> GPGYNEPMAASDEVNLIESRTVVPLNTWVLISNFKVAYNILRRPDGTFNRHLAEYLDRKVTANANPVDGVFSFDVLIDRRINLLSRVYRPAYADQEQPPSILDLEKPVDGDIVPVILFFHGGSFAHSSANSAIYDTLCRRLVGLCKCVVVSVNYRRAPENPYPCAYDDGWIALNWVNSRSWLKSKKDSKVHIFLAGDSSGGNIAHNVALRAGESGIDVLGNILLNPMFGGNERTESEKSLDGKYFVTVRDRDWYWKAFLPE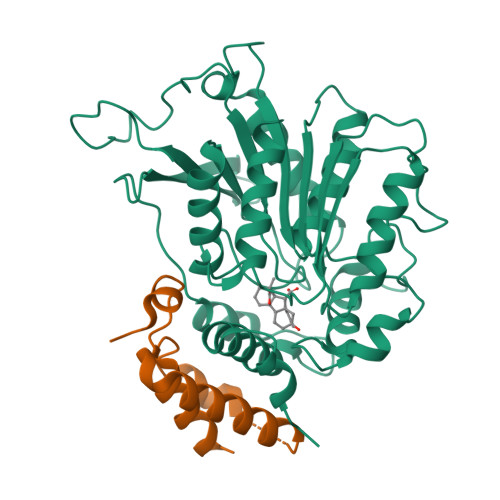GEDREHPACNPFSPRGKSLEGVSFPKSLVVVAGLDLIRDWQLAYAEGLKKAGQEVKLMHLEKATVGFYLLPNNNHFHNVMDEISAFVNAE;> GPGYNEPQDKKTMMMNEEDDGNGMDELLAVLGYKVRSSEMADVAQKLEQLEVMMSNVQEDDLSQLATETVHYNPAELYTWLDSMLTDLNPPSSNAEYDLKAIPGDAILNQ>[2x]MSAKKIVLKSSDGESFEVEEAVALESQTIAHMVEDDCVDNGVPLPNVTSKILAKVIEYCKRHVEAAASKAEAVEGAATSDDDLKAWDADFMKIDQATLFELILAANYLNIKNLLDLTCQTVADMIKGKTPEEIRTTFNIKNDFTPEEEEEVRRENQWAFE;>[2x]MAEEEEVEEGRSSSSAILDLPEPLLLHILSFLTDVRSRHRAALACGRMRAAERATRSELSLRGDPRSPGFLFLSHAFRFPALEHLDLSLVSPWGHPLLSSVPPCGGGGGGAPSASSSSGMNVYHPEAISEQNAFIAARLAGCFPAVTSLAVYCRDPTTLANLTPHWQASLRRVKLVRWHQRPPTLPDGADLEPLLETCAALRELDLSEFYCWTEDVVRALTTHPSATAALTHLDLGLAAATDGFKSSELGPIAASCPNLRKL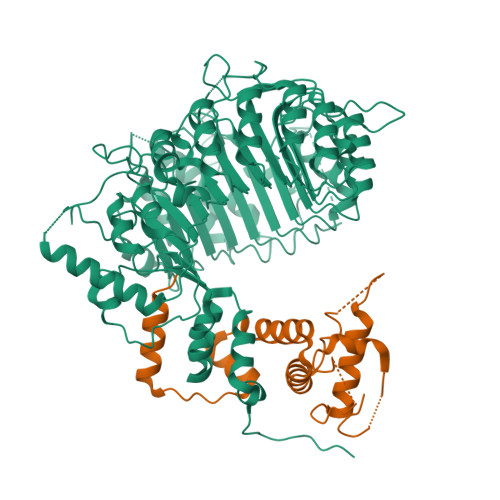VAPCLFNPRFSDCVGDDALLSLATSCPRLTVLRLSEPFEAAANIQREEAAITVAGLVAFFAALPALEDFTMDLQHNVLEAAPAMEALARRCPRIKFLTLGSFQGLCKASWLHLDGVAVCGGLESLYMKNCQDLTDASLAAIGRGCRRLAKFGIHGCDLVTSAGIRRLAFTLRPTLKEVTVLHCRLLHTAECLTALSPIRDRIESLEINCVWNTTENLYFQSLGSWEMLRSLSLWFSAGQLLSPLISAGLDSCPVLEEISIKVEGDCRTCPRPAPRTIFGLSDLAGFPVLAKMKLDLSEAVGYALTAPTGQMDLSLWERFYLHGIESLQTLYELDYWPPQDKDVHHRSLTLPAVGLIQRCVGLRKLFIHGTTHEHFMTFFLSIPNLRDMQLREDYYPAPENDLMFTEMRAESWLRFEVQLNSRQIDD>[3x]MSFFHASQRDALNQSLAEVQG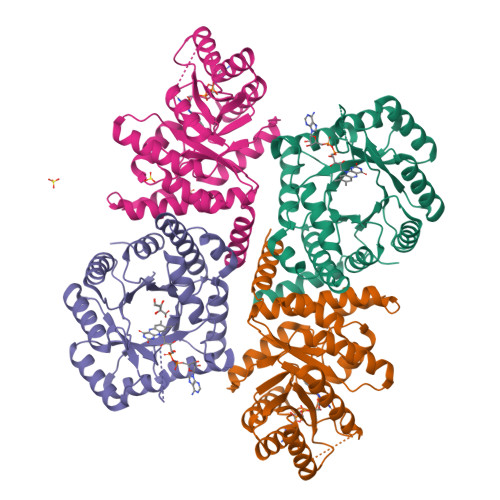QINVSFEFFPPRTSEMEQTLWNSIDRLSSLKPKFVSVTYGANSGERDRTHSIIKGIKDRTGLEAAPHLTCIDATPDELRTIARDYWNNGIRHIVALRGDLPPGSGKPEMYASDLVTLLKEVADFDISVAAYPEVHPEAKSAQADLLNLKRKVDAGANRAITQFFFDVESYLRFRDRCVSAGIDVEIIPGILPVSNFKQAKKLADMTNVRIPAWMAQMFDGLDDDAETRKLVGANIAMDMVKILSREGVKDFHFYTLNRAEMSYAICHTLGVRPGLLEHHHHHH~{N}-[(2-methylphenyl)methyl]-3-[(2-methylphenyl)methylamino]pyrazine-2-carboxamide | C21 H22 N4 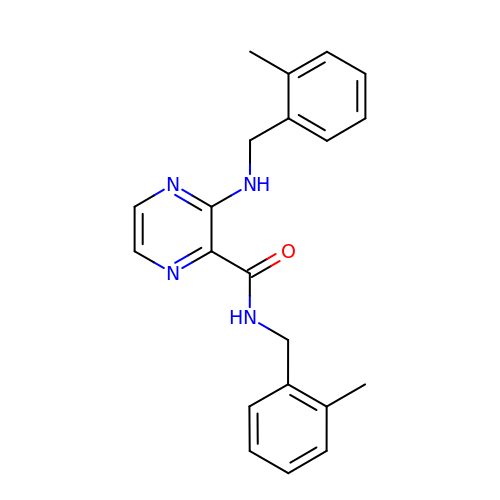O | HDTUPNYLSOQSAV-UHFFFAOYSA-N>MDQKQFEKIRAVFDRSGVALTLVDMSLPEQPVVLANPPFLRMTGYTEGQILGFNCRFLQRGDENAQARADIRDALKLGRELQVVLRNYRANDEPFDNLLFLHPVGGRPDAPDYFLGSQFELGRSGNSEEAAAAGHAGALTGELARIGTVAARL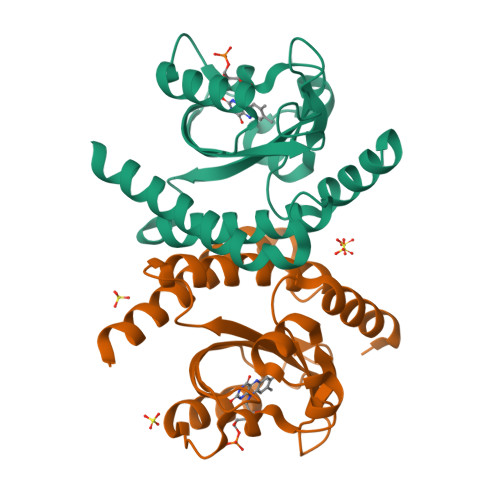EMDSRRHLAQAAAALVRAWERRG[2x]>[7x]HHHHHHSSGLVPRGSHMVVADTKSLKLLALADKVAKTDANVMILGPSGSGKEVMSRYIHNASPRKEGPFIAINCA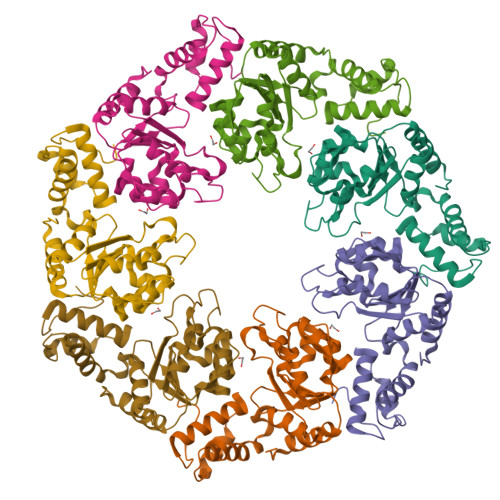AIPDNMLEATLFGYEKGAFTGAVQACPGKFEQAQGGTILLDEISEMDLNLQAKLLRVLQEREVERLGSRKSIKLDVRVLATSNRDLKQYVQAGHFREDLYYRLNVFPLTWPALCERKDDIEPLANHLIERHCKKLGLPVPSIAPNAITKLLNYPWPGNVRELDNVVQRALILSENGHIQSEHILLEGVDWHD> GPMKKIEAIVKPFKLDDVREALTEIGITGMTVSEVKGFGRQKGHTEIYRGAEYA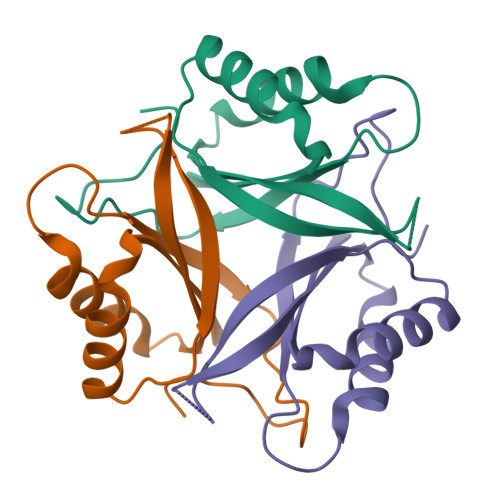VDFLPKIKIELVLADDAVERAIDVIVEVARSGKIGDGKIFVLPVEEAIRIRTGERSDAAV4-[[(2~{R},3~{S})-2-methylpiperidin-3-yl]amino]-2-phenyl-thieno[3,2-c]pyridine-7-carboxamide | C20 H22 N4 O S | 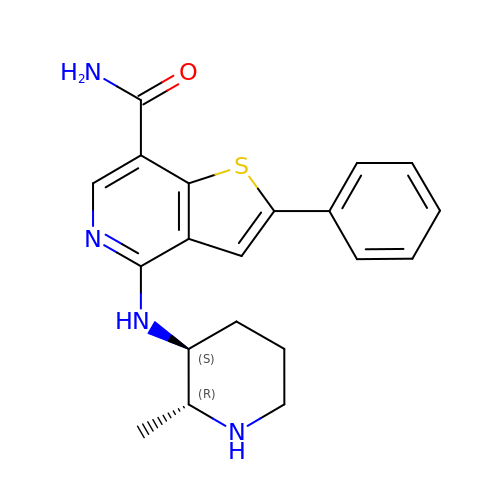LMQOZGSVTQQPFU-WBMJQRKESA-N>SIHMFPSDFKWGVATAAYQIEGAYNEDGRGMSIWDTFAHTPGKVKNGDNGNVACDSYHRVEEDVQLLKDLGVKVYRFSISWPRVLPQGTGEVNRAGLDYYHRLVDELLANGIEPFCTLYHWDLPQALQDQGGWGSRITIDAFAEYAELMFKELGGKIKQWITFNEPWCMAFLSNYLGVHAPGNKDLQLAIDVSHHLLVAHGRAVTLFRELGISGEIGIAPNTSWAVPYRRTKEDMEACLRVNGWSGDWYLDPIYFGEYPKFMLDWYENLGYK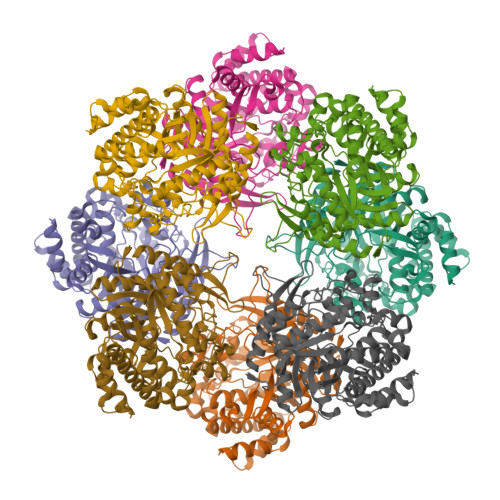PPIVDGDMELIHQPIDFIGINYYTSSMNRYNPGEAGGMLSSEAISMGAPKTDIGWEIYAEGLYDLLRYTADKYGNPTLYITENGACYNDGLSLDGRIHDQRRIDYLAMHLIQASRAIEDGINLKGYMEWSLMDNFEWAEGYGMRFGLVHVDYDTLVRTPKDSFYWYKGVISRGWLDL[16x]1,4-dideoxy-4-thio-nojirimycin 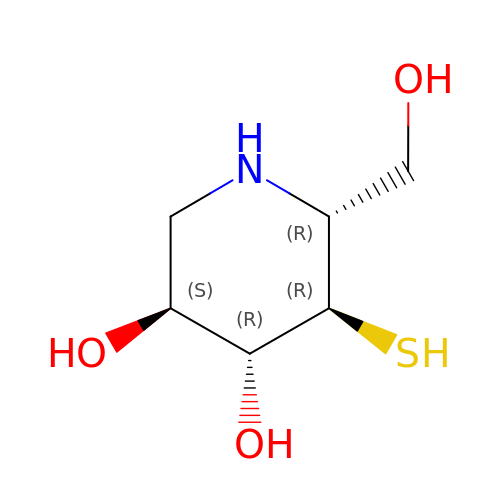| C6 H13 N O3 S | NSHHSUUKQHDEOL-JGWLITMVSA-N> MDVLIEWVAIYPQIYDILEHINYVPSNTLQRLRLHQPWSKIDYDVWFLYASDEIRETCKVKYYGETKTYGEVFVLENERISQLHRLFVSWTVSERAEHLKNLLFDAGLSNLPLVELGGNVFFNSHVPLPCSLVLTKSTQENLNRITPYLVQKRPILLAGPEGIGKKFLITQIAAKLGQQIIRIHLSDSTDPKMLIGTYTSPKPGEFEWQPGVLTQAVITGKWILFTNIEHAPSEVLSVLLPLLEKRQLVIPSRGETIYAKGSFQMFATSSMKTKILGQRLWQILDLTYQPDECVEVVSTLYPVLSIICPTLYSVYKDIFDLFSQRSFLATSKIYRRLCLRDFYKFIKRVAFLYHKFMIPSDHVVISQELQDAVFKEAIDMFGAFIPSRDGFDLVVRNVAIELNIPPEKALQLRYSIPVFQNLEHNINIGRCSLKKLSTIRSCSTNSYAFTSSSLGLLEQLAAGVQTNEPLLLVGETGTGKTTTIQLLAGLLGQKVTVINMSQQTESSDMLGGYKPINASTLGLPLHERFIDIFEQTFSSKKNAKFISMASTSARRFRWKTCLKIWKEACKLSKTVLDGQQPLPNPQKRQKRLSNQVELRNQWAKFEKEVEDFEKVLTGGSNGFMFSFVEGALVKAVRSGHWVLLDEINLASLETLEPIGQLLSSYESGILLSERGDITPITPHKNFRLFGCMNPSTDVGKRELEPSFRSRFTEIYVHSPDQNLDDLLSIIQKYIGSLCIGNEHVIREVAELYQVAKSLSLDGSLVDGAGQRPHYTVRTLSRTLSYVTEIAPIYGLRRSLYEGFCMSFLTLLDHTSESLLYNHVVRFTLGELNRDQQNAILKQIPKVPDHSSYIAFCHYWLRRGSFPVEEQEHYIITPFVQKNLLNIARACSTRMFPILIQGPTSSGKTSMIEYVAKKTGHKFVRINNHEHTDLQEYIGTYVTDDNGSLSFREGVLVEALRNGYWIVLDELNLAPTDVLEALNRLLDDNRELFIPETQVLVKPHPEFMLFATQNPPGVYAGRKHLSRAFRNRFLEIHFDDIPENELETILHKRCKIAPSYAAKIVQVFRELSLRRQTTRIFEQKNSFATLRDLFRWAFREAVGYQQLAENGYMLLAERARDQKDKLAVQEVIEKVMKVKIDTDGIYNLDSMEIFQDMSLKEGPLSKVVWTRPMIRLFCLVWRCLLAKEPVLLVGDTGCGKTTVCQILAECLHKELHIINAHQDTENGDIIGAQRPVRNRSAVNYSLHSQLCEKFNVQESLDSIDDLIEKFEKLSSSEKNDNLSNLIERQIIKYRSLFEWHDGALVTAMKQGDFFLLDEISLADDSVLERLNSVLELSRTLTLVEHSNAAVSLTAKDGFAFFATMNPGGDYGKKELSPALRNRFTEIWVPPMVDTEDILKIVEGKLHNNKIELARPLVEYAKWHANEYLYTDVISIRDVLSAVEFINACEILDLNLVLFNAVSMVFIDALGSFTTFSLSNNLASLHAERQRCFAKLNELAGSNIMASKSADISIKFSDSSFFIGDFGIPLGDSVESDSTYSLHTDTTLMNASKVLRALQVLKPILLEGSPGVGKTSLITALARETGHQLVRINLSDQTDLMDLFGSDVPVEGGEGGQFAWRDAPFLAAMRNGHWVLLDELNLASQSVLEGLNACLDHRNEAYIPELDKVFKAHPNFRVFAAQNPQHQGGGRKGLPRSFINRFSVVYVEALKEKDMIEIAACNYHQVNEDWRLKIIKFMFRLQDNIEKDISFGSFGSPWEFNLRDTLRWLQLLNDAPKYTCVSPADYLEVMVLHRMRTVEDRVRTCELFKEVFDIDYEPRTIGFSLSSQCFKVGHSLLVRDVERQKTLLDSQNILQSQLPVLESVITCINKKWPCILVGDTATGKTCILRLLAAIAGAKIKEMAVNSDTDTMDLIGEYEQIDISRKASELFTDLSQQLLNIVIKYRNFDNIFRETSLYTLTTTSFKTHSQAFTLLQKVVDQLDQLKIHETLVHSLGDIHEKARKLLAEFSASPAGRFEWFDGYLLKAVEEGHWFVLDNANLCSPAVLDRLNSLLEHKGVLIVNEKTTEDGHPKTIKPHPNFRLFLTVNPVYGELSRAMRNRGVEIFLLKEALTEIDKKQMSLLEPAPISSAVDTLASNISYIKYVFETMGKIEIDGNYMYIAHAIILALFSPRQLKLLRKVLLTNPQFSLSIKADAELLLTLKNLVQKIYCADYFNHMDLKASRFMDIYEYPVQLREVVGLIQTINDFQSVILTSHLELPETYASGLLFVSAHEILDLTEEVNRLAVSTSNSTYLLKSASAVYHNVSSFKGSTPSLWNLLNQFSKFLIEIASANSNIVYKLSYDVIRHFLKLVVLWKNIYVWTNVPDCDISRFYCYTKMLGEWMFTLTEKTKLLESFLPKDSLEKFSELQNLSTGLHMQAIWDKWHAFVPRTYDQWSLWNTVDKLLTQYVNANIPSISMETTACEVVGTSLSLLNKVLVENEVGDIYSYLKILGKGVNELKSSKQVILPENLVNLFNCLASLDLLHIFIKYTTSSFFLTDDFVRFIRVCFHSRISGNLLTLLHGISFDSTKAVAPVLTYFDFCSLTTGNILGRIALAFTSIDENANLESANIFEHARLALLQHFMDHSSLLAEDSSTKMNL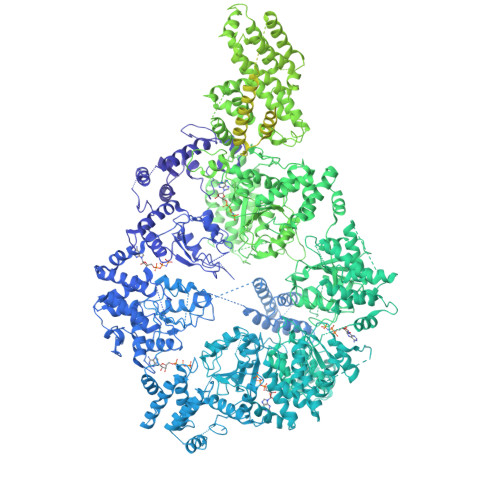ILLQRYAVIISIFLDQGKCEKANDLITKLSLPYEELAENFVSILEACKAFLVANSEFISYTYTERFIHSLRFLKDSWLSSNQQKMLKNQGMAYIYFASGMLLVYVPDKPFDPALLPLLTVESLRHYLESLYKESQILEIAESLNSGKVNSVMRRLVSTEISNTPNIDSSFSTVYRSLNESIVPLYSELEFFMKSVVLNQYIFELAMRLSKESNIAVVEEAKSFVTKWKAYIERIREAYPQFVDVYELILSFISFMIYGIELLMFEAKRRLDERSQILSTLILTLVDPSSFARSLSFDDVSNLIEQIKVLDLNDSIRFEIYLFLASRLCSEKQHSSDTHSLANSFVLLANEFYIHNAKIKQKELEEIEEKNRLYRQREFNFDKNDYLKVFINYDDEVEPEVEPEVVIERKRFLQLQFAFWSLYNEIYSEKMNVIPLEQLMNTGSYLAKKIKVKNPDMIASSGFDIVSVVLMMGVKSTNERQYWTPPVYNFYSDPNPSKAIEVRDLIKIVESRAISLIKNWPENFVLRGLKDAIDAILNLSPFSPIAEYLSKLERVFHLLSEWEKLASREYSLANEMDLIKKKIIDWRKFELSNWNNLLKLEEYKLSERVYPRLYSILQFIILKPFFENSKFTKQNLCESASIIVQFITDLTVGEFQLCLKCLLSFSQHAASLRICHGIDAMLLNIYHYFEQFLSKVSEAIHTQKQSLENSIKERILLMSWKDTNVYALKESAKKSHAELFKVLHRYREVLRQPVSSYLSQKHDWDSLLDTENNSAMWVAKKVNLSPSYIEKMDTEIMKLVPVRFSNTPTTLRLMWTLFANVEKPGSTFTNMVSNLITDARELMKLTPETINDDNLSEIKHLKSRKHLLLTETFKTLKAFGLQYRVKAGIEENLSNLRNLLAVIPTFPVTSLSIEKVDRSLMKSLDFIPKFQTLAGHQHNDLSVPEVQKGVGLFNSMLSLQLGERAQLVEFTNELLALKNVYSEVGVNGSPLESFNNSSFNEVSSLGYDHDFENRAQAVSMLCQIYAIVIQKHSSISPTASFQSIGHELSRFADLLSNKLFPSSIPLYASADKVSSIRDQQKGINDLIEYCRKKRTELPELSYCFKHLVSLQSLKSISRTQVDLTNDEFLNLMNFVLNLFDSLLSSIETATKNMRTFKELAETSSFIEMSSCFSKVLRAFNLKFQSMKLSSLKEKLRSSSVDKMSCQLLMLFLPVCEQFINLAESVLDYFINVHNSNLDSLSKISTLFFMVANNGFCSPDLPQEGKSNSGELESGTGLGSGVGAEDITNTLNEDDDLEELANEEDTANQSDLDESEARELESDMNGVTKDSVVSENENSDSEEENQDLDEEVNDIPEDLSNSLNEKLWDEPNEEDLLETEQKSNEQSAANNESDLVSKEDDNKALEDKDRQEKEDEEEMSDDVGIDDEIQPDIQENNSQPPPENEDHLDLPEDLKLDEKEGDVSKDSDLEDMDMEAADENKEEADAEKDEPMQDFEDPLEENNTLDEDIQQDDFSDLAEDDEKMNEDGFEENVQENEESTEDGVKSDEELEQGEVPEDQAIDNHPKMDAKSTFASAEADEENTDKGIVGENEELGEEDGAAESGVRGNGTADGEFSSAEQVQKGEDTSTPKEAMSEADRQYQSLGDHLREWQQANRIHEWEDLTESQSQAFDDSEFMHVKEDEEEDLQALGNAEKDQIKSIDRDESANQNPDSMNSTNIAEDEADEVGDKQLQDGQDISDIKQTGEDTLPTEFGSINQSEKVFELSEDEDIEDELPDYNVKITNLPAAMPIDEARDLWNKHEDSTKQLSIELCEQLRLILEPTLATKMQGDFRTGKRLNMKRIIPYIASQFKKDKIWMRRVKPSKRTYQVMISIDDSKSMSESGSTVLALETLALVTKALSLLEVGQIAVMKFGEQPELLHPFDKQFSSESGVQMFSHFTFEQSNTNVLALADASMKCFNYANTASHHRSNSDIRQLEIIISDGICEDHDSIRKLLRRAQEEKVMIVFVILDNVNTQKKSSILDIKKVYYDTKEDGTMDLKIQPYIDEFAFDYYLVVRNIEELPQLLSSALRQWFQQMSNT>[2x]MSFIPVAEDSDFPIQNLPYGVFSTQSNPKPRIGVAIGDQILDLSVIKHLFTGPALSKHQHVFDETTLNNFMGLGQAAWKEARASLQNLLSASQARLRDDKELRQRAFTSQASATMHLPATIGDYTDFYSSRQHATNVGIMFRGKENALLPNWLHLPVGYHGRASSIVVSGTPIRRPMGQMRPDNSKPPVYGACRLLDMELEMAFFVGPGNRFGEPIPI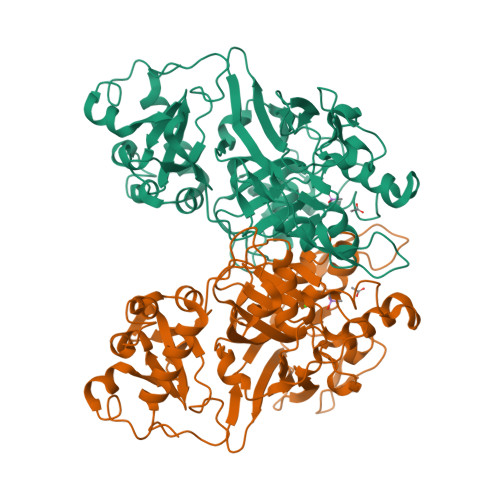SKAHEHIFGMVLMNDWSARDIQQWEYVPLGPFLGKSFGTTISPWVVPMDALMPFVVPNPKQDPKPLPYLCHSQPYTFDINLSVSLKGEGMSQAATICRSNFKHMYWTMLQQLTHHSVNGCNLRPGDLLASGTISGSDPESFGSMLELSWKGTKAIDVGQGQTRTFLLDGDEVIITGHCQGDGYRVGFGQCAGKVLPALSPA As an FAD-dependent hydroxylase, 4-hydroxyphenylacetate 3-hydroxylase (HpaB) is able to ortho-hydroxylate phenylpropanoids in a molecular chaperon-independent manner and has broad substrate specificity and high catalytic activity. Among them, the HpaBC complex from E. coli (EcHpaBC) has outstanding activities and a broad substrate spectrum. More interestingly, we found that EcHpaB is also capable of hydroxylating a series of phenylpropanoids to generate a wide range of natural products. The highest titers were reported at 62.7 mg/L and 34.7 mg/L in whole-cell catalysis studies, respectively. These results indicate that EcHpaB has a broad substrate spectrum for the hydroxylation of a variety of phenolic compounds.

In this study, we solved the crystal structure of EcHpaB apoenzyme for the first time by X-ray crystallography. EcHpaB is an (α2)2 tetramer, the model consists of residues 2–519 for each of the four-polypeptide chains in the crystallographic asymmetric unit. The N-terminal (MHHHHHHHK) purification tags (residues −7 to 0), Met 1 and the Lys 520 for each chain were not observed in the electron density maps and were excluded from the final model. The tetramer can best be described as dimer of homodimers with chains A and B forming one dimer and chains C and D forming the other. The overall EcHpaB structure contains 30 helices and 16 β strands, which make up five β sheets. Interestingly, the low-homology sequences of EcHpaB and TtHpaB enzymes results in highly similar three-domain architecture and 3-dimensional structure. Structural alignment of EcHpaB and TtHpaB revealed a distinct sequence and structural difference in the loop connecting strands β32 and β33 and covering the entrance of the catalytic site, which consists of eleven amino acids. However, based on the secondary structure prediction, the EcHpaB β32-β33 loop appears to be segmented into three sections, two random coils were separated by a Type IV β-turn. In contrast, the corresponding loop in TtHpaB is a simple random coil. In all cases the crude modeling suggested that the EcHpaB active site could accommodate these substrates in part owing to the plasticity of the β32-β33 loop and the observation that main chain hydrogen bonding to loop residues played a key role in positioning the substrate in the active site.

>[4x]MHHHHHHHKPEDFRASTQRPFTGEEYLKSLQDGREIYIYGERVKDVTTHPAFRNAAASVAQLYDALHKPEMQDSLCWNTDTGSGGYTHKFFRVAKSADDLRQQRDAIAEWSRLSYGWMGRTPDYKAAFGCALGANPGFYGQFEQNARNWYTRIQETGLYFNHAIVNPPIDRHLPTDKVKDVYIKLEKETDAGIIVSGAKVVATNSALTHYNMIGFGSAQVMGENPDFALMFVAPMDADGVKLISRASYEMVAGATGSPYDYPLSSRFDENDAILVMDNVLIPWENVLIYRDFDRCRRWTMEGGFARMYPLQACVRLAVKLDFITALLKKSLECTGTLEFRGVQADLGEVVAWRNTFWALSDSMCSEATPWVNGAYLPDHAALQTYRVLAPMAYAKIKNIIERNVTSGLIYLPSSARDLNNPQIDQYLAKYVRGSNGMDHVQRIKILKLMWDAIGSEFGGRHELYEINYSGSQDEIRLQCLRQAQNSGNMDKMMAMVDRCLSEYDQDGWTVPHLHNNDDINMLDKLLK N1-(3-(2-(6-Amino-4-methylpyridin-2-yl)ethyl)-5-fluorophenyl)-N1-cyclopropyl-N2-methylethane-1,2-diamine | C20 H27 F N4 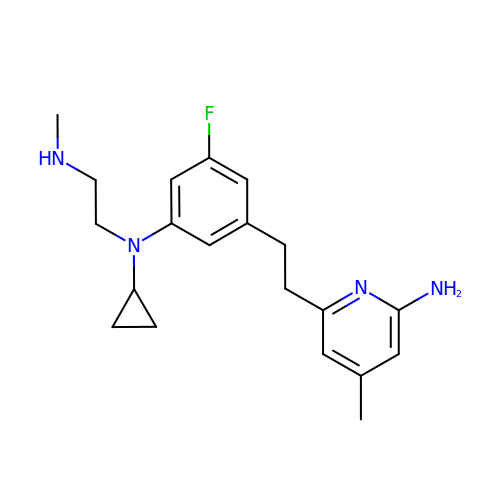| CZBLKBKVAIKTJH-UHFFFAOYSA-N> GPTIYHAKDAVQATKPDMRKPRLVVFVVGETARADHVSFNGYERDTF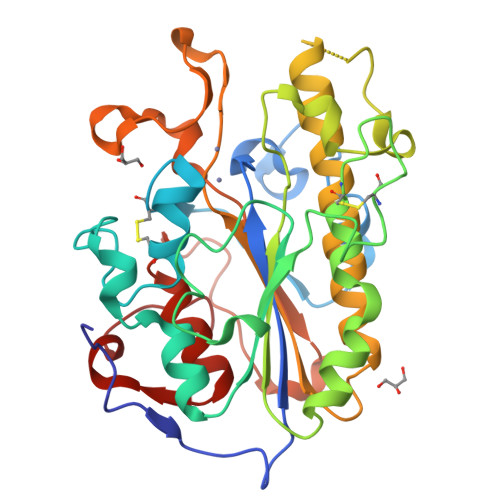PQLAKIDGVTNFSNVTSCGTSTAYSVPCMFSYLGADEYDVDTAKYQENVLDTLDRLGVSILWRDNNSDSKGVMDKLPKAQFADYKSATNNAICNTNPYNECRDVGMLVGLDDFVAANNGKDMLIMLHQMGNHGPAYFKRYDEKFAKFTPVCEGNELAKCEHQSLINAYDNALLATDDFIAQSIQWLQTHSNAYDVSMLYVSDHGESLGENGVYLHGMPNAFAPKEQRSVPAFFWTDKQTGITPMATDTVLTHDAITPTLLKLFDVTADKVKDRTAFIR> MGSDKIHHHHHHENLYFQGRDKPLVFFNRQPSDPLTGKVDMAAMNWNDKTYYVGFDAKFGGSIQGKMILDFLASSESSVDRNGDGIIGYVLCIGDVGHNDSKVRTEGIRRALGTWTGSSDPGQAKEGQAVVGGKSYKVVELEGKAMTGTDGSTWNTNSATESMGSWVAKFADKIDLVISNNDGMAMGCLQASNYPRGLPIFGYDANADAVESVGKGELTGTVSQNVDAQAVAVLQIIRNLLDGSSGEDVVANGISRPDAHGNKISAPVQYWEDVKAIMADNSEVTSANWKEYTRGARDAGVRQVSAPTKKVLLTVHNASNDFLASAYLPALKHYAPLLNVDLTVVQGDGQNELSCLDKFTNLDMFDAFAVNMVKTNSGADYTDKLKY

In this report, we found that TpMglB-2, the product of gene tp0684, is very likely the D-glucose-binding protein of an ABC transporter dedicated to the import of this vital molecule. The overall fold of TpMglB-2 resembles those of LBPs (sometimes called “Periplasmic Binding Proteins”) that serve as receptors for nutrients and cofactors in bacterial ABC transporters. LBPs generally have two structurally similar lobes that are attached by a hinge region. TpMglB-2 has an unconventional topology for an LBP, but retains the hallmarks of ligand binding and ligand-induced conformational change that are common to this family of proteins.

Purified, recombinant TpMglB-2 readily formed crystals that diffracted X-rays to a minimum Bragg spacing of 2.05 Å. The final model after refinement featured excellent geometry, and 366 of the 387 residues present in the construct were visible in the electron-density maps. The large cleft region is solvent-accessible, and thus this structure of TpMglB-2 appears to be in the “open” conformation. The first is a calcium ion, which is located at the far end of the lobe, about 30 Å distant from the cleft. This cation is coordinated by atoms from four side chains of TpMglB-2: D71, N73, D75, and D166. The Ca2+ appears to stabilize a loop on the C lobe while simultaneously adhering it to the main body of the domain. The second small molecule is located in the interlobe cleft in association with residues of the C lobe; it is BIS-TRIS, which had been included in both the crystallization medium and the cryoprotection buffer at a concentration of 100 mM. Hydrogen bonds to hydroxyl groups on the buffer molecule are provided by the side chains of residues D91, R95, N172, and D195, and an additional van der Waals interaction is made by the side chain of H89. Although this site likely overlaps with the ligand-binding site (see below), the fact that TpMglB-2 adopts an open conformation with this small molecule bound suggests that its binding is adventitious. Comparisons of the structures of TpMglB-2 and EcMglB also reveal a stark difference in the proteins: their topologies are circularly permuted. The hinges of Type I/Cluster B LBPs are usually made up of three regions of irregular secondary structure representing points where the primary structure crosses over from one lobe to the other. The permutation noted above in TpMglB-2 necessitates a fourth cross-over; this region of the protein (residues 284–288) is close to the canonical hinge.>[8x]MSKIAPQCQNLREQVNQLIELLRQEPTLRSQQDTSIVETALGKALSPRFEIVFAGAFSAGKSMLINALLERELLYSAEGHATGTECHIEYANANEERVVLTFLSEAEIRQQALILAKYLNVNVGDLNINQPEAVKVVSQYCQKIIAEEGGENKSERAKQANALHLLLIGFEQNRERINTVQNSTYSMDQLN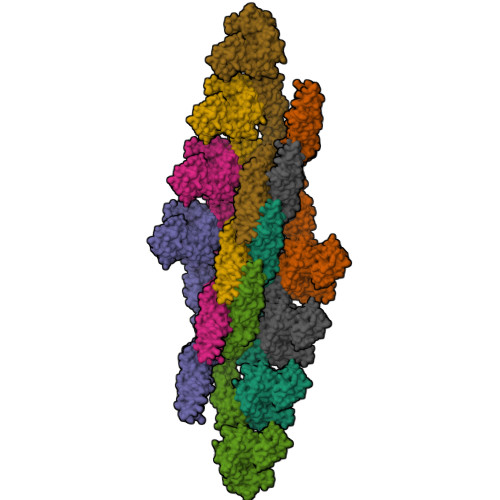FSSLAEAAGYARRGANSAVLKRLDYFCNHSLLKDGNVLVDLPGIDAPVKEDAERAYRKIESPDTSAVICVLKPAAAGDMSAEETQLLERISKNHGIRDRVFYVFNRIDDTWYNTQLRQRLEGLIQSQFRDNSRVYKTSGLLGFYGSQVKQTNSSTRFGLDSIFATTIKGFDGEEETPQFVSEFNNYCANSGKLLSTAFRVSVNGYETSNENYVRILSEWGIPLVDQLIHDSGIESFRSGIGLYLAEEKYPELFATLANDLQPLCIALRQFYLENYRQLDSQPREIAAMKAQELTLLNQEMQNLGIEFKKYMSAQINDVVIGNDREFDQDFTKLKARMVARLDELLKTFSVMNAYKRATESHPRNSTAPFIAVLVEALYYLANELEDAFIEAIHELVKNFFQRLGDRLRKVDCYHQVYRLVGNDGGIEQLLRRAEEDITKALVNEARTECDRYVRESPRFYDEGTFSIYQFRQTLQQTSQGYDAQAIVEAEPAIKELLKLDFEPKVFNTVRKNFRQTVNNTLKTHLLPMAEEQAQIILEQYDVARKYREQTLEQDAEEKIARNSRLQSEIKQKIDLYQTSIVSINECLKAMQIFEQLPVITESDITKQAEIVADADFVEIVELEHHHHHH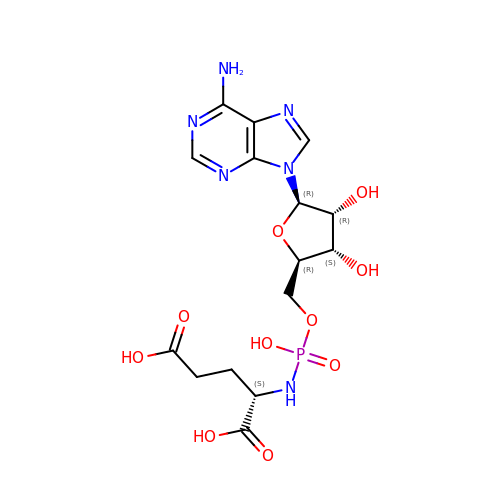(2S)-2-{[(S)-{[(2R,3S,4R,5R)-5-(6-amino-9H-purin-9-yl)-3,4-dihydroxyoxolan-2-yl]methoxy}(hydroxy)phosphoryl]amino}pentanedioic acid (non-preferred name) | C15 H21 N6 O10 P | CKTPKDBUYLAONN-LTOLZBHSSA-N> MAQINASYQRDMAIALPGMVADTSKYNIDGACVVNEGDVLVGAAVQVVQAQAVDGHKLVKALTTGTTPYGVAIRSHWQTVNAQNQMIYEDGGAINVMTSGRVWMLSKSTEAPTFGSAVK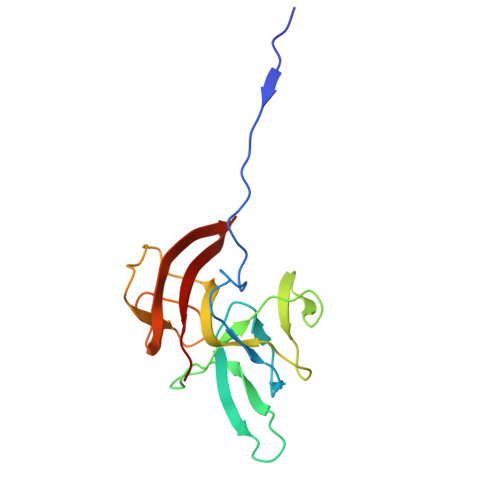LDVDGQEKSDGTIETTWTYAGGWTKYKDIQLVEVQLHQL> GSAKDPMNSEQQQTVFLCVSYLLSYPDEQWAESLPDCLDAIRSLDDETVRAPLLAVAEQLAITPARERMEQYVETFDFGKKTNLYLTYMTNGEQRERGIELVALKARYEAAGFAVSDHELPDYLPLMLEWMAYADQEHTTALL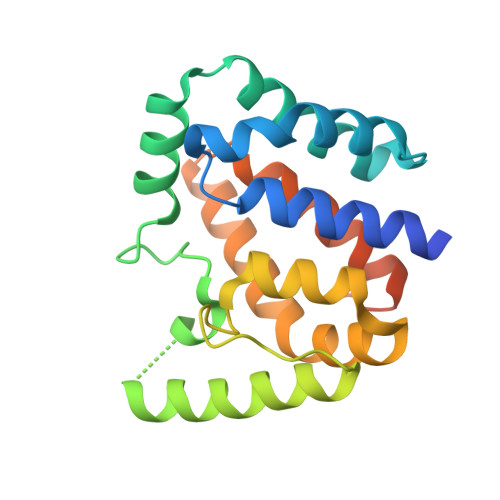ADYAGHIREIGDRLAAAGSPYAQLFDALNHTFTQLGVTPLPKGGATAWPANFSG>[4x]MQFRSIIRIVGLLLALFSVTMLAPALVALLYRDGAGVPFVTTFFVLLFCGAMCWFPNRRHKHELKSRDGFLIVVLFWTVLGSAGSLPFLIADNPNISVTDAFFESFSALTTTGATVIVGLDELPKAILFYRQFLQWFGGMGIIVLAVAILPVLGIGGMQLYRAEIPGPVKDTKMTPRIAETAKALWYIYLSLTIACAVAFWLAGMTPFDAISHSFSTIAIGGFSTHDASMGYFDSYAINLITVVFLLISACNFTLHFAAFASGGVHPKYYWKDPEFRAFIFIQVLLFLVCFLLLLKHHSYTSPYDAFDQALFQTVSISTTAGFTTTGFADWPLFLPVLLLFSSFIGGCAGSTGGGMKVIRILLLTLQGARELKRLVHPRAVYTIKVGGSALPQRVVDAVWGFFSAYA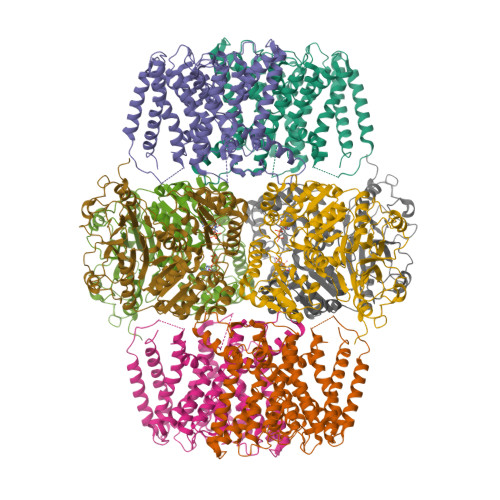LVFVVCMLGLIATGMDELSAFSAVAATLNNLGPGLGEVALHFGDVNDKAKWVLIVSMLFGRLEIFTLLILLTPTFWRS;>[4x]MKIIILGAGQVGGTLAENLVGENNDITIVDNNADRLRELQDKYDLRVVNGHASHPDVLHEAGAQDADMLVAVTNTDETNMAACQVAFTLFNTPNRVARIRSPEYLAEKEALFKSGAIPVDHLIAPEELVTSYIERLIQYPGALQVVSFAEQKVSLVAVKAYYGGPLVGNALSALREHMPHIDTRVAAIFRQGRPIRPQGTTIIEADDEVFFVAASNHIRSVMSELQRLEKPYRRIMIVGGGNIGASLAKRLEQTYSVKLIERDYQRAEKLSEQLENTIVFCGDAADQELLTEENIDQVDVFIALTNEDETNIMSAMLAKRMGAKKVMVLIQRGAYVDLVQGGVIDVAISPQQATISALLTHVRRADIVNVSSLRRGAAEAIEAVAHGDETTSKVVGRAIGDIKLPPGTTIGAVVRGEEVLIAHDRTVIEQDDHVVMFLVDKKYVPDVEALFQPSPFFL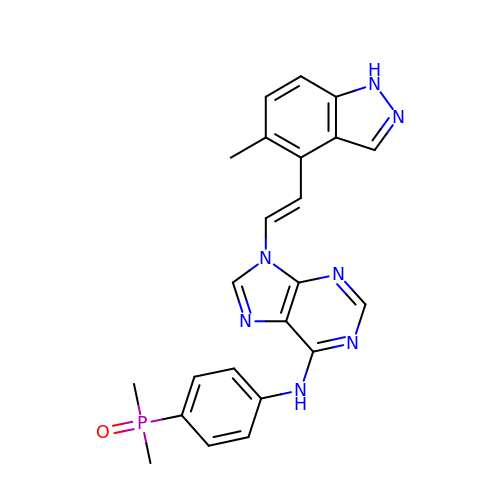N-[4-(dimethylphosphoryl)phenyl]-9-[(E)-2-(5-methyl-1H-indazol-4-yl)ethenyl]-9H-purin-6-amine | C23 H22 N7 O P | UNPSONVHRMUXFE-ZHACJKMWSA-N>[2x]MDEELYTLIEFLKKPSISATGEGIDETANYLKETVEKLLGVKANLEKTKGHPVVYAEINVNAKKTLLIYNHYDVQPVDP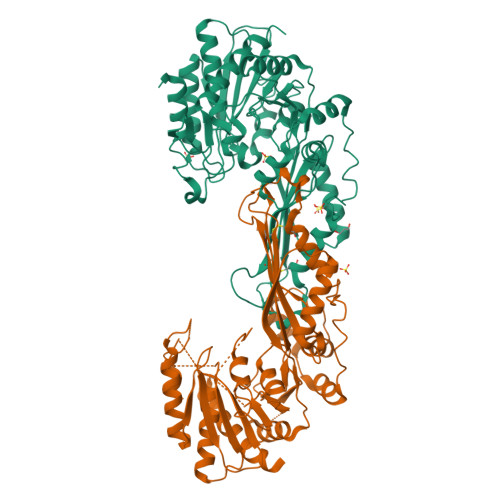ISEWKRAPFSATIENDRIYARGASDNKGTLMARLFAIKHLLDKNELNVNVKLLYEGEEEIGSVNLEDYIEKNTNKLKADSVIMEGAGLDPKGRPQIVLGVKGLLYVELVLDYGTKDLHSSNAPLVRNPCIDLAKIISTLVDMGGRVLIEGFYDDVRELTEEERELIKKYDIDVEELKKALGFKELKYNEKEKIAEALLTYPTCNVDGFECGYTGKGSKTIVPHRAFAKLDFRLVPNQDPYKVFELLKKHLQKAGFNGEILAHGFEYPVRTSVNSTVVKAMIESAKKVYGTEPQVIPNSAGTQPMGLFVYKLGIRDAVSAIGAGGYYSNAHAPNENIKIDDYYKAIKHTEEFLKLYPIL> MPELRPILLVEDNPRDLELTLTALEKCQLANEVVVARDGTEALDYLNVTGSYHNRPGGDPAVVLLDLKLPKVDGLEVLQTVKG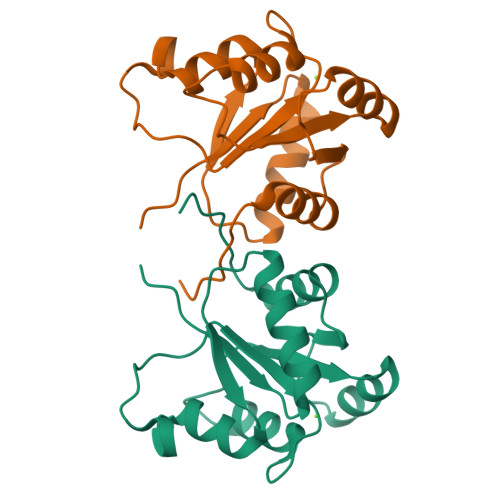SDHLRHIPVVMLTSSREEQDLVRSYELGVNAFVVKPVEFNQFFKAIQDLGVFWALLNE> GPMAAASGSVLQRCIVSPAGRHSASLIFLHGSGDSGQGLRMWIKQVLNQDLTFQHIKIIYPTAPPRSYTPMKGGISNVWFDRFKITNDCPEHLES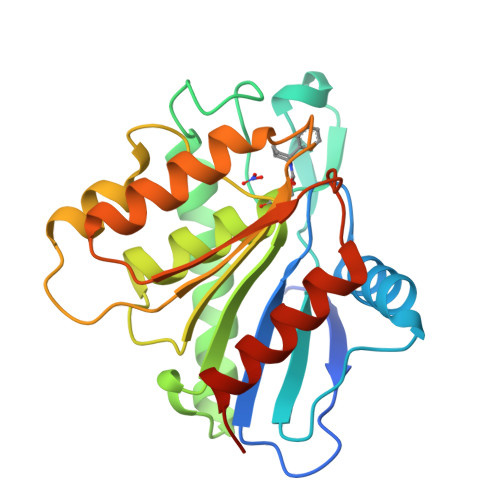IDVMCQVLTDLIDEEVKSGIKKNRILIGGFSMGGCMAMHLAYRNHQDVAGVFALSSFLNKASAVYQALQKSNGVLPELFQCHGTADELVLHSWAEETNSMLKSLGVTTKFHSFPNVYHELSKTELDILKLWILTKLPGEMEKQK>EIPLKYGATNEGKRQDPAMQKFRDNRLGAFIHWGLYAIPGGEWNGKVYGGAAEWLKSWAKVPADEWLKLMDQWNPTKFDAKKWAKMAKEMGTKYVKITTKHHEGFCLWPSKYTKYTVANTPYKRDILGELVKAYNDEGIDVHFYFSVMDWSNPDYRYDIKSKEDSIAFSRFLEFTDNQLKELATRYPTVKDFWFDGTWDASVKKNGWWTAHAEQMLKELVPGVAINSRLRADDKGKRHFDSNGRLMGDYESGYERRLPDPVKDLKVTQWDWEACMTIPENQWGYHKDWSLSYVKTPIEVIDRIVHAVSMG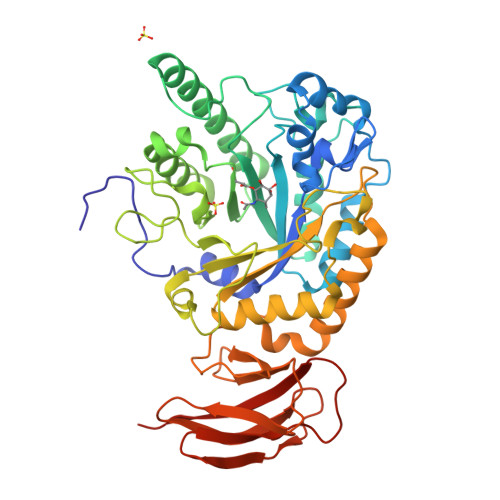GNMVVNFGPQADGDFRPEEKAMATAIGKWMNRYGKAVYACDYAGFEKQDWGYYTRGKNDEVYMVVFNQPYSERLIVKTPKGITVEKATLLTTGEDITVVETTRNEYNVSVPKKNPGEPYVIQLKVRAAKGTKSIY[4x]>[2x]ANPLYQKHIISINDLSRDDLNLVLATAAKLKANPQPELLKHKVIASCFFEASTRTRLSFETSMHRLGASVVGFSDSANTSLGKKGETLADTISVISTYVDAIVMRHPQEGAARLATEFSGNVPVLNAGDGSNQHPTQTLLDLFTIQETQ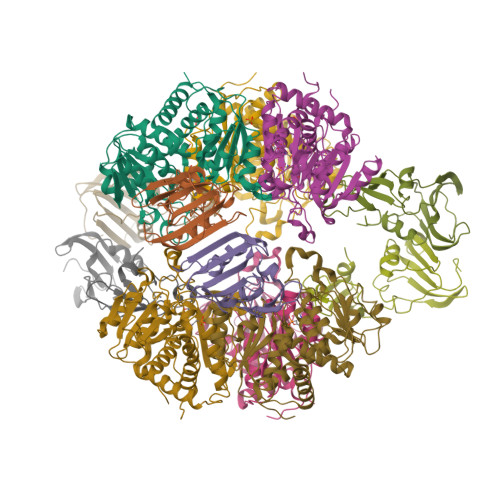GRLDNLHVAMVGDLKYGRTVHSLTQALAKFDGNRFYFIAPDALAMPQYILDMLDEKGIAWSLHSSIEEVMAEVDILYMTRVQKERLAPSEYANVKAQFVLRASDLHNAKANMKVLHPLPRVDEIATDVDKTPHAWYFQQAGNGIFARQALLALVLNRDLVL;>MTHDNKLQVEAIKRGTVIDHIPAQIGFKLLSLFKLTETDQRITIGLNLPSGEMGRKDLIKIENTFLSEDQVDQLALYAPQATVNRIDNYEVVGKSRPSLPERIDNVLVCPNSNCISHAEPVSSSFAVRKRANDIALKCKYCEKEFSHNVVLAN[2x]>HHHHHHTDRFTRLLGIQQPIIQAPMLGVSTPALAAAVSNAGGLGSIAITGSAAEKGRALIREVRGLTDKPFNVNLFCHRPGQADPARERAWLDYLKPLFAEFGAEPPVRLKNIYLSFLEDPTLLPMLLEERPAAVSFHFGAPPRDQVRALQAVGIRVLVCATTPEEAALVEAAGADAVVAQGIEAGGHRGVFEPERGDAAIGTLALVRLLAARGSLPVVAAGGIMDGRGIRAALELGASAVQMGTAFVLCPESSANAAYREALKGPRAARTALTVTMSGRSARGLPNRMFFDAAAPGVPPLPDYPFVYDATKALQTAALARG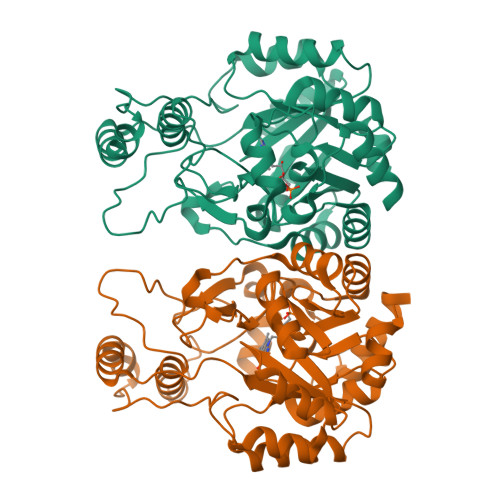NHDFAAQWAGQGAALARELPAAELLRTLVEELRG[2x]>MIVLALDVYEGERAIKIAKSVKDYISMIKVNWPLILGSGVDIIRRLKEETGVEIIADLKLADIPNTNRLIARKVFGAGADYVIVHTFVGRDSVMAVKELGEIIMVVEMSHPGALEFINPLTDRFIEVANEIEPFGVIAPGTRPERIGYIRDRLKEGIKILAPGIGAQGGKAKDAVKAG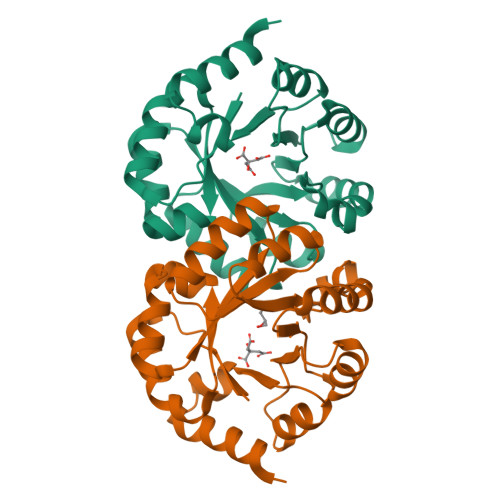ADYIIVGRAIYNAPNPREAAKAIYDEIRGV[2x]> SLAKRIIAALDVKDGRVVKGTNFENLRDSGDPVELGKFYSEIGIDELVFHDHTASVEKRKTMLELVEKVAEQIDIPFTVGGGIHDFETASELILRGADKVSINTAAVENPSLIT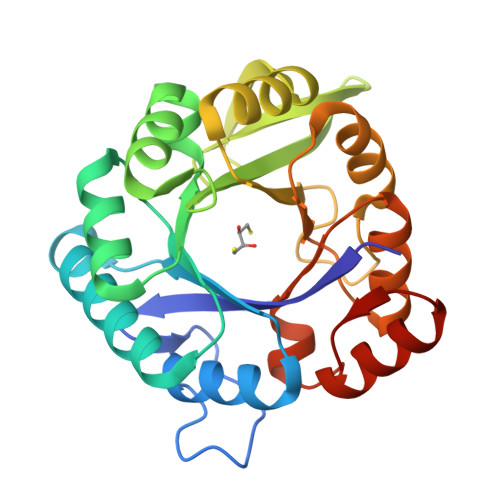QIAQTFGSQAVVVAIDAKRVDGEFMVFTYSGKKNTGILLRDWVVEVEKRGAGEILLTSIDRDGTKSGYDTEMIRFVRPLTTLPIIASGGAGKMEHFLEAFLAGADAALAASVFHFREIDVRELKEYLKKHGVNVRLEGL>SNYVAKVNTLETEEWFFKDITRKDAERQLLAPGNSAGAFLIRESETLKGSFSLSVRDYDPMHGDVIKHYKIRSLDNGGYYISPRITFPCISDMIKHYQK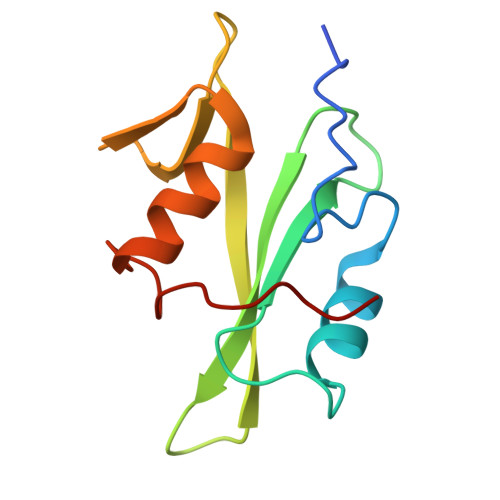QSDGLCRRLEKACISP[2x]>[6x]YEHTAVMPNKVGIPYKALVERPGYAPVHLQIQLVNTRIIPSTNLEYITCKYKTKVPSPVVKCCGATQCTSKPHPDYQCQVFTGVYPFMWGGAYCFCDTENTQMSEAYVERSEECSIDHAKAYKVHTGTVQAMVNITYGSVSWRSADVYVNGETPAKIGDAKLIIGPLSSAWSPFDNKVVVYGHEVYNYDFPEYGTGKAGSFGDLQSRTSTSNDLYANTNLKLQRPQAGIVHTPFTQAPSGFERWKRDKGAPLNDVAPFGCSIALEPLRAENCAVGSIPISIDIPDAAFTRISETPTVSDLECKITECTYASDFGGIATVAYKSSKAGNCPIHSPSGVAVIKENDVTLAESGSFTFHFSTANIHPAFKLQVCTSAVTCKGDCKPPKDHIVDYPAQHTESFTSAISATAWSWLKVLVGGTSAFIVLGLIATAVVALVLFFHRH;>DLDTHFTQYKLARPY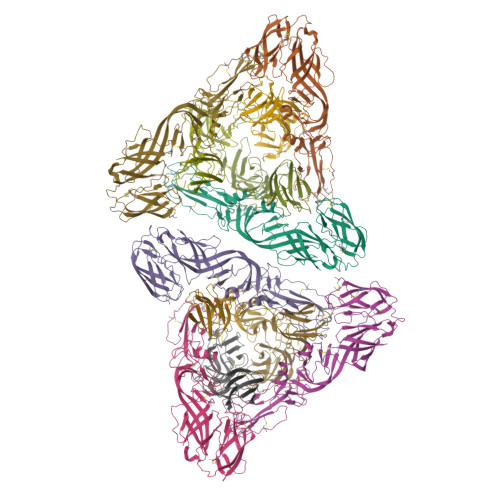IADCPNCGHSRCDSPIAIEEVRGDAHAGVIRIQTSAMFGLKTDGVDLAYMSFMNGKTQKSIKIDNLHVRTSAPCSLVSHHGYYILAQCPPGDTVTVGFHDGPNRHTCTVAHKVEFRPVGREKYRHPPEHGVELPCNRYTHKRADQGHYVEMHQPGLVADHSLLSIHSAKVKITVPSGAQVKYYCKCPDVREGITSSDHTTTCTDVKQCRAYLIDNKKWVYNSGRLPRGEGDTFKGKLHVPFVPVKAKCIATLAPEPLVEHKHRTLILHLHPDHPTLLTTRSLGSDANPTRQWIERPTTVNFTVTGEGLEYTWGNHPPKRVWAQESGEGNPHGWPHEVVVYYYNRYPLTTIIGLCTCVAIIMVSCVTSVWLLCRTRNLCITPYKLAPNAQVPILLALLCCIKPTRA[6x]(2S)-({[2-(5-cyano-3-hydroxypyridin-2-yl)-1,3-thiazol-4-yl]acetyl}amino)(phenyl)ethanoic acid | C19 H14 N4 O4 S | 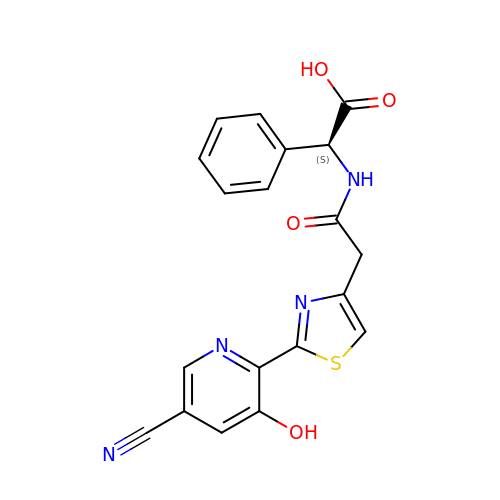KPGRSPXHOOAVBE-INIZCTEOSA-N>MAHHHHHHMYAIGLTGGIGSGKTTVADLFAARGASLVDTDLIAHRITAPAGLAMPAIEQTFGPAFVAADGSLDRARMRALIFSDEDARRRLEAITHPLIRAETEREARDAQGPYVIFVVPLLVESRNWKARCDRVLV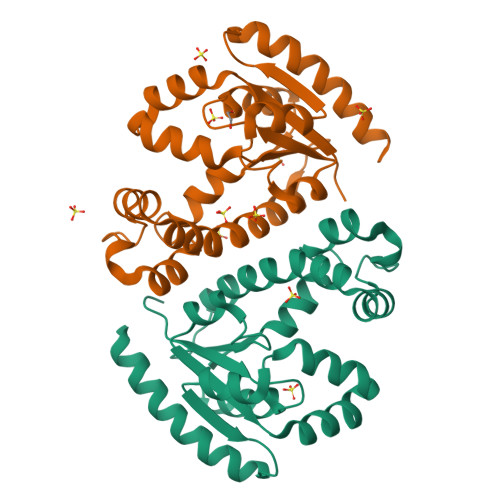VDCPVDTQIARVMQRNGFTREQVEAIIARQATREARLAAADDVIVNDAATPDALAVQVDALHQRYLAFAAAKH[2x]N-(6-chloro-3,3-dimethyl-3,4-dihydroisoquinolin-1-yl)-3-[2-propyl-4-(1H-pyrazol-4-yl)thiophen-3-yl]-L-alanine | C24 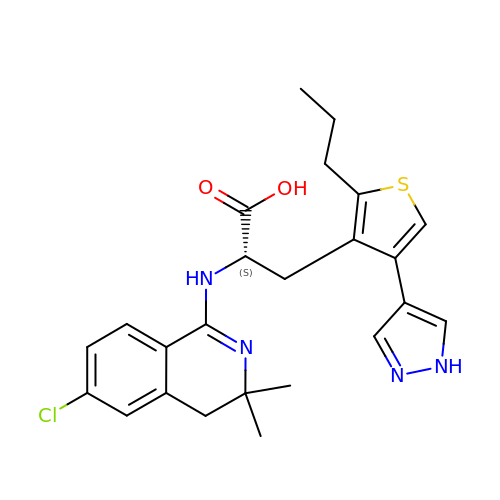H27 Cl N4 O2 S | GZLUSHWHRPZJDJ-FQEVSTJZSA-N> SEVSDTNLYSPFKPRNYQLELALPAMKGKNTIICAPTGCGKTFVSLLICEHHLKKFPNGQKGKVVFFANQIPVYEQNKSVFSKYFERHGYRVTGISGATAENVPVEQIVENNDIIILTPQILVNNLKKGTIPSLSIFTLMIFDECHNTSKQHPYNMIMFNYLDQKLGGSSGPLPQVIGLTASVGVGDAKNTDEALDYICKLCASLDASVIATVKHNLEELEQVVYKPQKFFRKVESRISDKFKYIIAQLMRDTESLAKRICKDLENLSQIQNREFGTQKYEQWIVTVQKACMVFQMPDKDEESRICKALFLYTSHLRKYNDALIISEHARMKDALDYLKDFFSNVRAAGFDEIEQDLTQRFEEKLQELESVSRDPSNENPKLEDLCFILQEEYHLNPETITILFVK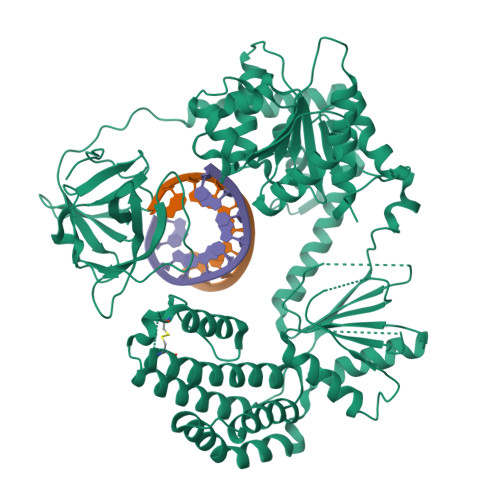TRALVDALKNWIEGNPKLSFLKPGILTGRGKTNQNTGMTLPAQKCILDAFKASGDHNILILTSVADEGIDIAQCNLVILYEYVGNVIKMIQTRGRGRARGSKCFLLTSNAGVIEKEQINMYKEKMMNDSILRLQTWDEAVFREKILHIQTHEKFIRDSQEKPKPVPDKENKKLLCRKCKALACYTADVRVIEECHYTVLGDAFKECFVSRPHPKPKQFSSFEKRAKIFCARQNCSHDWGIHVKYKTFEIPVIKIESFVVEDIATGVQTLYSKWKDFHFEKIPFDPAEMSK>GSHMERPRQIRQLRAALQSLEAEIMYGHTPLHTASQQIAKQLAQPVSTLFSAFSDQLDKGSDSAKTAWEQSLKKVWDTLSLKKSEYEVLKQFG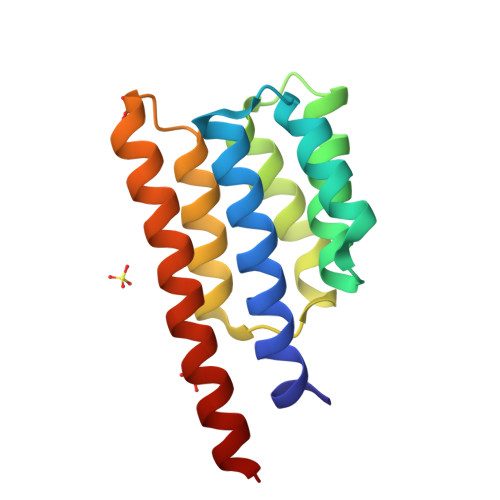ETLGIHDRISQQKHIKLALTHLEASEADAEQAQAKNE[4x]> MHHHHHHPEIVDTCSLASPASVCRTKHLHLRCSVDFTRRTLTGTAALTVQSQEDNLRSLVLDTKDLTIEKVVINGQEVKYALGERQSYKGSPMEISLPIALSKNQEIVIEISFETSPKSSALQWLTPEQTSGKEHPYLFSQCQAIHCRAILPCQDTPSVKLTYTAEVSVPKELVALMSAIRDGETPDPEDPSRKIYKFIQKVPIPCYLIALVVGALESRQIGPRTLVWSEKEQVEKSAYEFSETESMLKIAEDLGGPYVWGQYDLLVLPPSFPYGGMENPCLTFVTPTLLAGDKSLSNVIAHEISHSWTGNLVTNKTWDHFWLNEGHTVYLERHICGRLFGEKFRHFNALGGWGELQNSVKTFGETHPFTKLVVDLTDIDPDVAYSSVPYEKGFALLFYLEQLLGGPEIFLGFLKAYVEKFSYKSITTDDWKDFLYSYFKDKVDVLNQVDWNAWLYSPGLPPIKPNYDMTLTNACIALSQRWITAKEDDLNSFNATDLKDLSSHQLNEFLAQTLQRAPLPLGHIKRMQEVYNFNAINNSEIRFRWLRLCIQSKWEDAIPLALKMATEQGRMKFTRPLFKDLAAFDKSHDQAVRTYQEHKASMHPVTAMLVGKDLKVD

LTA4H (EC 3.3.2.6) is a bifunctional zinc-containing enzyme that catalyzes the conversion of the labile LTA4 epoxide to the pro-inflammatory and immune-modulating lipid mediator, leukotriene B4 (LTB4). In addition to the epoxide hydrolase activity, LTA4H also catalyzes the peptidolytic inactivation of a chemotactic tripeptide, Pro-Gly-Pro (PGP). The elucidation of high-resolution crystal structures of LTA4H revealed the binding mode of LTA4 and PGP in the L-shaped substrate channel with overlapping active sites. The channel can be divided into two parts: the wider polar region containing the substrate entry site and catalytic center, and the narrower hydrophobic tunnel accommodating long fatty acid tails.

In the current project, new inhibitors, 4-(4-benzylphenyl) selenazol-2-amine (TTSe) and 4-(4-benzylphenyl) oxazole-2-amine (TTO) were synthesized based on the lead compound, ARM1. Specifically, the sulphur atom in the thiazole ring of ARM1 was replaced with other chalcogens, namely selenium or oxygen, resulting in the selenazole and oxazole derivatives, TTSe and TTO, respectively. Similarly to ARM1, TTSe and TTO bound to the end of the hydrophobic substrate channel and interact with the polypeptide chain of LTA4H via hydrogen–hydrogen interactions. In addition, the hydrophilic moiety of TTSe and TTO was coordinated by two water molecules connected with the peptide bonds of A377 and S379 from one side or D312 and W315 from the other side. The hydrophilic selenazole or oxazole ring can rotate via a single C-C bond; therefore, densities of two rotamers are detected. TTSe and TTO-bound LTA4H structures are in a closed conformation which is in accordance with stabilizing conformational changes observed with DSF. The binding of inhibitors results in the conformational rotations of Y383 and Y378 which together with catalytic Zn2+ coordinate the substrate for efficient catalysis. The Ki values for ARM1, TTSe and TTO with LTA4H were 1.5, 4.8 and 3.8 µM, respectively. Similarly to ARM1, TTSe and TTO did not influence the cleavage of the PGP tripeptide by recombinant LTA4H. In addition, it should be noted that ARM1 and TTSe do not affect the activity of recombinant soluble epoxide hydrolase (sEH) activity, whereas TTO at higher concentrations may affect metabolism of fatty acid epoxides.> MSDVTQQKKRKRSKGEVNPSKPTVDEEITDPS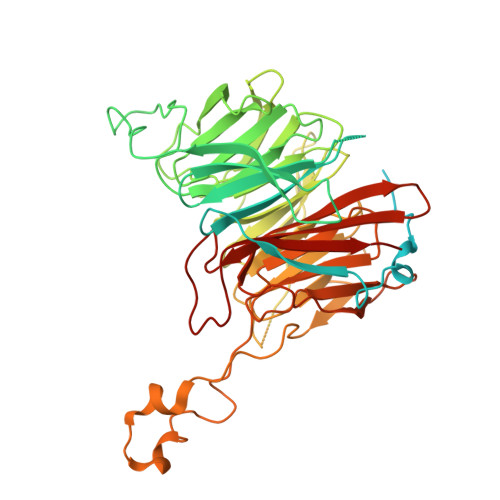SNEDEQLEVSDEEDALESEEEFEGENPADKRRRLAKQYLENLKSEANDILTDNRNAEEKDLNNLKERTIDEYNNFDAGDLDKDIIASRLKEDVAEQQGRVFRYFGDKLLISEAKQSFTRVGENNLTCISCFQPVLNKYTFEESSNGDKNKGRLFAYTVSKDLQLTKYDITDFSKRPKKLKYAKGGAKYIPTSKHEYENTTEGHYDEILTVAASPDGKYVVTGGRDRKLIVWSTESLSPVKVIPTKDRRGEVLSLAFRKNSDQLYASCADFKIRTYSINQFSQLEILYGHHDIVEDISALAMERCVTVGARDRTAMLWKIPDETRLTFRGGDEPQKLLRRWMKENAKEGEDGEVKYPDESEAPLFFCEGSIDVVSMVDDFHFITGSDNGNICLWSLAKKKPIFTERIAHGILPEPSFNDISGETDEELRKRQLQGKKLLQPFWITSLYAIPYSNVFISGSWSGSLKVWKISDNLRSFELLGELSGAKGVVTKIQVVESGKHGKEKFRILASIAKEHRLGRWIANVSGARNGIYSAVIDQTGF>[8x]MRTRIFIGSSKEGLKEANYVKSRLEKANFEVFIWNDDIFKPNKNTLETLLNVASLFDFGIMIATKDDFTASRDDIFETVRDNVVFEFGLFLGRLGENRAFALQENGAKLPSDLLGITIPKFEKTDDYFSNYNLNTEIDNIIKIINEKISLGELGLLPSTVLAIGYYENFVSTVCDALHSLPTIKLNGIEYKDFVFNIIIPNDLDADIKRRAQIYFKKMDIHEVKIDTNGRSFPLYLQIDEENSGDVAVLYDMPTTLGGIDKAIEMYMKKGHIGKTSQQQLLEERELRNFKTTLINLINNNSFTKTFVKVIEE

CBASS operons encode cyclic dinucleotide synthases (CD-NTases) and effector proteins (Caps), such as bacterial STING, which senses cyclic dinucleotides like 3′3′-c-di-GMP to trigger defense. Here, we resolve cryo-EM structures of Epilithonimonas lactis TIR-STING (ElSTING) bound to 3′3′-c-di-GMP, revealing two oligomeric states: spiral-shaped single filaments and fiber bundles composed of straight protofibrils. The overall structure of the ElSTING dimer closely resembles that of the SfSTING dimer, comprising an N-terminal TIR domain and a C-terminal STING domain, connected by a linker. Functional assays confirmed that 3′3′-c-di-GMP is the sole CDN capable of activating ElSTING-mediated NAD+ degradation, cleaving NAD+ into ADP-ribose (ADPr) and nicotinamide (NAM) as observed in SfSTING homologs.

The structure of the fiber bundle was resolved at 3.7 Å resolution. The packing of the ElSTING fiber bundle is mediated by the TIR domain, with each protofibril rotating approximately 22.5° to its neighboring protofibril. In contrast to the spiral architecture of ElSTING single filaments, protofibrils within the ElSTING fiber bundle adopt a straight configuration, mirroring the linear assembly observed in SfSTING filaments. Notably, the interactions between the TIR domains of protofibrils contribute to their assembly. Specifically, F128 within the DD loop of one TIR domain packs against residues Y19 and F128 of a neighboring domain. By contrast, in the protofibril structure, the two guanine rings move closer, transforming the U-shaped 3′3′-c-di-GMP into a Δ-shaped conformation. Although F39 remains buried, upward displacement of the CBDα4 helix disrupts its interactions with the hydrophobic core, likely permitting NAD+ binding to trigger F39 flipping and active site assembly. Notably, residue Q278 occupies the site which was previously held by the calcium ion, while residues K269 and K274 establish charge-charge interactions with E264 and E282, respectively. Collectively, these structural and mechanistic parallels confirm that the ElSTING fiber bundle represents its active form, underscoring the role of conformational dynamics in STING-mediated activation.> VGVSGSAEGFAKGVTGGGSATPVYPDTIDELVSYLGDDEARVIVLTKTFDFTDSEGTTTGTGCAPWGTASACQVAIDQDDWCENYEPDAPSVSVEYYNAGTLGITVTSNKSLIGEGSSGAIKGKGLRIVSGAENIIIQNIAVT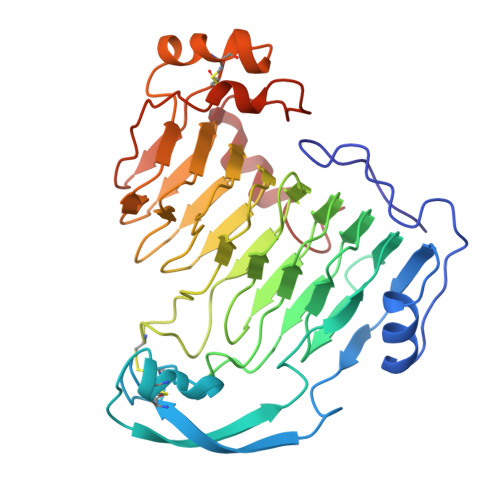DINPKYVWGGDAITLDDCDLVWIDHVTTARIGRQHYVLGTSADNRVSLTNNYIDGVSDYSATCDGYHYWAIYLDGDADLVTMKGNYIYHTSGRSPKVQDNTLLHAVNNYWYDISGHAFEIGEGGYVLAEGNVFQNVDTVLETYEGEAFTVPSSTAGEVCSTYLGRDCVINGFGSSGTFSEDSTSFLSDFEGKNIASASAYTSVASRVVANAGQGNL> AV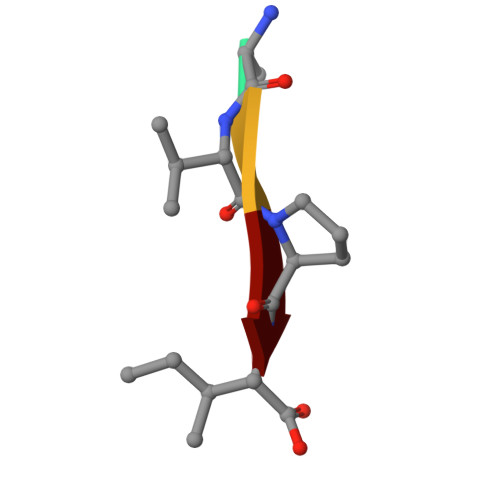PI(2E,4E,6E,8E,10E)-11-[(4R)-4-hydroxy-2,6,6-trimethylcyclohex-1-en-1-yl]-5,9-dimethylundeca-2,4,6,8,10-pentaenal | C22 H30 O2 | 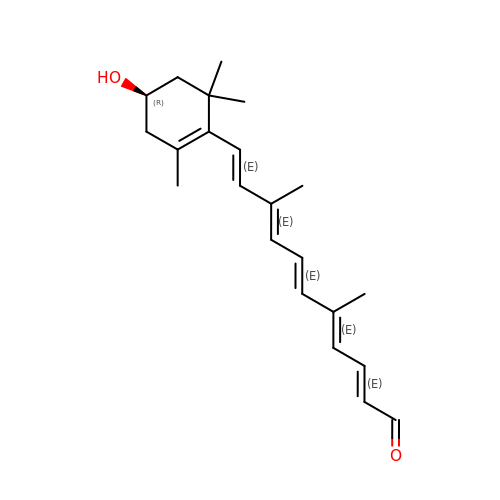BCNPTKKIVMTZFO-UWYNECTCSA-N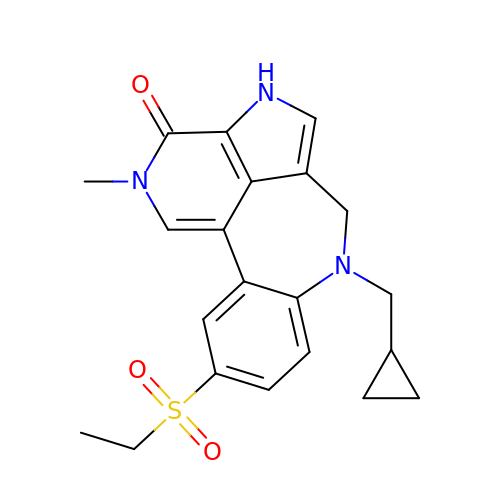7-(cyclopropylmethyl)-10-(ethylsulfonyl)-2-methyl-2,4,6,7-tetrahydro-3H-2,4,7-triazadibenzo[cd,f]azulen-3-one | C21 H23 N3 O3 S | RZNRQDHAAUZMFW-UHFFFAOYSA-N>GHMGNGKSIAGDQKAVPTQETHVWYRTFMMEYPSGLQTLHEFKTLLGLQGLNQKANKHIDQVYNTFDTNKDGFVDFLEFIAAVNLIMQEKMEQKLKWYFKLYDADGNGSIDKNELLDMFMAVQALNGQQTLSPEEFINLVFHKIDINNDGELTLEEFINGMAKDQDLLE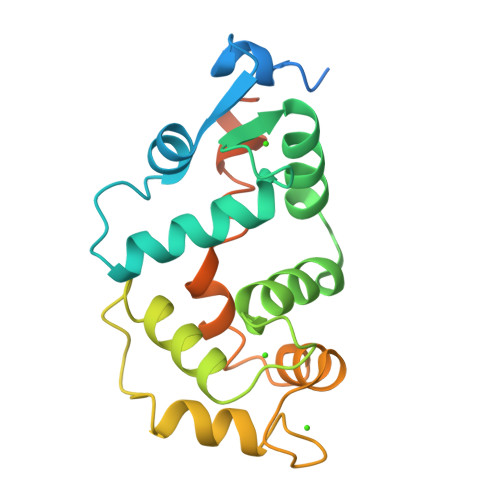IVYKSFDFSNVLRVICNGKQPDMETDSSKSPDKAGLGKVKMK[2x]>[12x]STRFTEEYQLFEELGKGAFSVVRRCVKVLAGQEYAAKIINTKKLSARDHQKLEREARICRLLKHPNIVRLHDSISEEGHHYLIFDLVTGGELFEDIVAREYYSEADASHCIQQILEAVLHCHQMGVVHRDLKPENLLLASKLKGAAVKLADFGLAIEVEGEQQAWFGFAGTPGYLSPEVLRKDPYGKPVDLWACGVILYILLVGYPPFWDEDQHRLYQQIKAGAYDFPSPEWDTVTPEAKDLINKMLTINPSKRITAAEALKHPWISHRSTVASCMHRQETVDCLKKFNARRKLKGAILTTMLATRNFSGGKSGGNKKSDGVKESSESTNTTIEDEDTKVRKQEIIKVTEQLIEAISNGDFESYTKMCDPGMTAFEPEA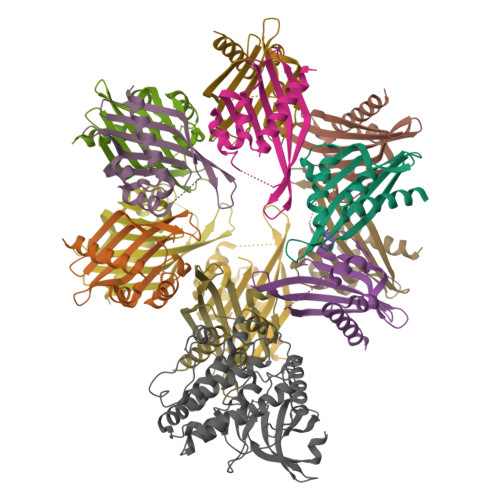LGNLVEGLDFHRFYFENLWSRNSKPVHTTILNPHIHLMGDESACIAYIRITQYLDAGGIPRTAQSEETRVWHRRDGKWQIVHFHRSGAPSVLPH;> STRFTEEYQLFEELGKGAFSVVRRCVKVLAGQEYAAMIINTKKLSARDHQKLEREARICRLLKHPNIVRLHDSISEEGHHYLIFDLVTGGELFEDIVAREYYSEADASHCIQQILEAVLHCHQMGVVHRNLKPENLLLASKLKGAAVKLADFGLAIEVEGEQQAWFGFAGTPGYLSPEVLRKDPYGKPVDLWACGVILYILLVGYPPFWDEDQHRLYQQIKAGAYDFPSPEWDTVTPEAKDLINKMLTINPSKRITAAEALKHPWISHRSTVASCMHRQETVDCLKKFNARRKLKGAILTTMLATRNFSGGKSGGNKKSDGVKESSESTNTTIEDEDTKVRKQEIIKVTEQLIEAISNGDFESYTKMCDPGMTAFEPEALGNLVEGLDFHRFYFENLWSRNSKPVHTTILNPHIHLMGDESACIAYIRITQYLDAGGIPRTAQSEETRVWHRRDGKWQIVHFHRSGAPSVLPH>[9x]MASHLASIYGTEQDKVNCSFYYKIGACRHGERCSRKHVKPNFSQTILCPNMYKNPIHEPNGKKFTQRELAEQFDAFYEDMFCEFSKYGEVEQLVVCDNVGDHLVGNVYVRFKYEESAQNAIDDLNSRWYSQRPVYAELSPVTDFREACCRQHETSECQRGGLCNFMHAKKPSPQLLRDLVLAQRKYLALNAAEEMKKEPNSDST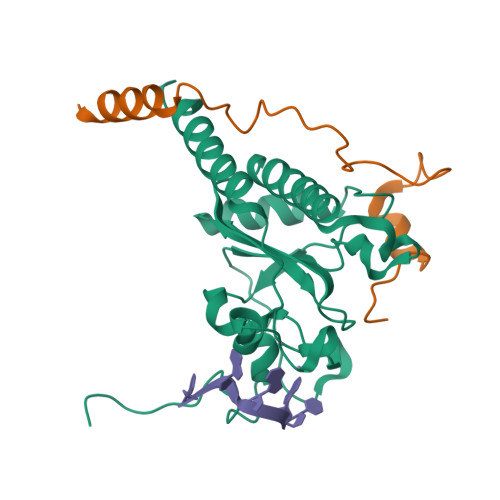NRWVSVTAERKN;>SSVGRSRSPPPSRERSVRSIEQELEQLRDVTPINQWKRKRSLWDIKPPGYELVTADQAKMSGVFPLPGA[9x]>MSVVQLNDENFDEVIKKNNKVVVVDFWAEWCGPCRMIAPIIEELAKEYAGKVVFGKLNVDENPEIAAKYG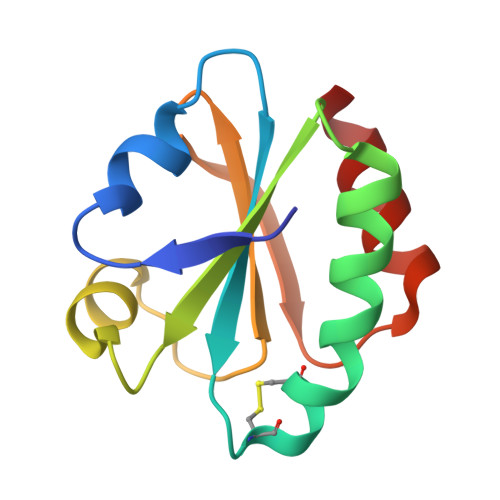IMSIPTLLFFKNGKVVDQLVGAMPKEALKERIKKYL[2x]> MRRSVYLDNTIEFLRGRVYLGAYDYTPEDTDELVFFTVEDAIFYNSFHLDFGPMNIGHLYRFAVIFHEILNDPENANKAVVFYSSASTRQRANAACMLCCYMILVQAWTPHQVLQPLAQ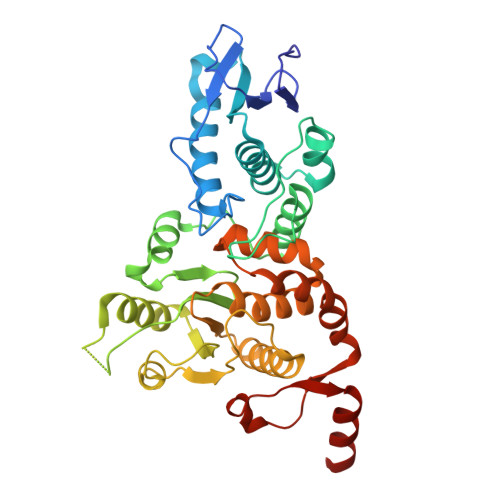VDPPFMPFRDAGYSNADFEITIQDVVYGVWRAKEKGLIDLHSFNLESYEKYEHVEFGDFNVLTPDFIAFASPQEDHPKGYLATKSSHLNQPFKSVLNFFANNNVQLVVRLNSHLYNKKHFEDIGIQHLDLIFEDGTCPDLSIVKNFVGAAETIIKRGGKIAVHCKAGLGRTGCLIGAHLIYTYGFTANECIGFLRFIRPGMVVGPQQHWLYLHQNDFREWKYTTRISLKPSEAIGGLYPLISLEEYRLQKKKLKD> MEEVRHIPVKSIIPNRFQPRTMFDEEKIDELALTIRTHGIIQPIVVRECGNGRFEIIAGERRWRAVQKLGWTEIPAIIKNLNDKETASVALIENLQREELTPIEEAMAYAKLIELHDLTQEALAQRLGKGQSTIANKLRLLKLPQEVQEALLQRAITERHARALIA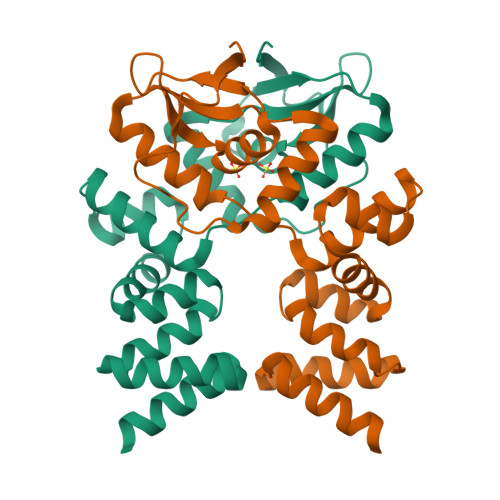LKDKEKQLKLLQEIIDKQLNVKQTEDRVLKLLEAGERKPKPKRKAFSRDKLAAALEHHHHHH>KPIEIIGAPFSKGQPRGGVEKGPAALRKAGLVEKLKETEYNVRDHGDLAFVDVPNDSPFQIVKNPRSVGKANEQLAAVVAETQKNGTISVVLGGDHSMAIGSISGHARVHPDLCVIWVDAHTDINTPLTTSSGNLHGQPVAFLLKELKGKFPDVPGFSWVTPCISAKDIVYIGLRD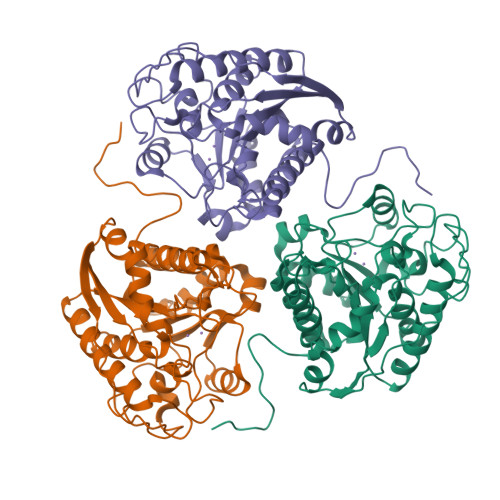VDPGEHYIIKTLGIKYFSMTEVDKLGIGKVMEETFSYLLGRKKRPIHLSFCVDGLDPVFTPATGTPVVGGLSYREGLYITEEIYKTGLLSGLDIMEVNPTLGKTPEEVTRTVNTAVALTLSCFGTKREGNHKPETDYL[3x]> QSESYKDAYSRINAIVIEGEQEAFDNYNRLAEMLPDQRDELHKLAKMEQRHMKGFMACGKNLSVTPDMGFAQKFFERLHENFKAAAAEGKVVTCLLIQSLIIECFAIAAFNIYIPVADAFARKITEGVVRDEYLHRNFGEEWLKANFDASKAELEEANRQNLPLVWLMLNEVADDARELGMERESLVEDFMIAYGEALENIGFTTREIMRMSAYG;> SYKDAYSRINAIVIEGEQEAFDNYNRLAEMLPDQRDELHKLAKMEQRHMKGFMACGKNLSVTPDMGFAQKFFERLHENFKAAAAEGKVVTCLLIQSLIIECFAIAAFNIYIPVADAFARKITEGVVRDEYLHRNFGEEWLKANFDASKAELEEANRQNLPLVWLMLNEVADDARELGMERESLVEDFMIAYGEALENIGFTTREIMRMSAYG

Cyanobacterial aldehyde-deformylating oxygenase (cADO), which catalyzes the conversion of Cn fatty aldehyde to its corresponding Cn-1 alk(a/e)ne, is a key enzyme in that pathway. Cyanobacterial aldehyde-deformylating oxygenase (cADO) belongs to the superfamily of ferritin-like di-iron proteins and contains a di-iron center. To gain insights into the reaction catalyzed by cADO, we determined structures of wild type ADO from Synechococcus elongates PCC7942 (Se) with different treatment (WT0, no treatment; WT1, co-crystallized with iron; WT-HP, soaked in H2O2), and solved the structures of two SeADO mutants (Y122F and F86YF87Y). SeADO belongs to the di-iron protein family, with conserved sequence of two EX28-29EX2H motifs, in which six conservative amino acids from four helices (Glu32 from helix H1, Glu115 from helix H4, Glu60 & His63 from helix H2, and Glu144 & His147 from helix H5) act as metal ligands.

In the Y122F structure, very little electron density was observed in the substrate channel, which is in contrast to all other four structures. However, there is still a little electron density remaining in the vicinity of the di-iron site, which we assigned to a water molecule forming a hydrogen-bond interactions with the carboxylic oxygen atoms of Glu144 and Glu115. This water molecule is not coordinated to either iron ions, with a distance of 3.28 Å and 3.15 Å, respectively. Apart from harboring the vacant substrate channel, the Y122F mutant shows comparable enzymatic activity with wild type. This result is consistent with that of the equivalent Y135F mutant in PmADO. In the Y122F structure, the di-iron site is surrounded by the four-helix bundle, each iron ion is penta-coordinated by two bridging carboxylates ligands (Glu60 and Glu144), one bidentate carboxylates and one histidine ligand (Glu32 and His63 for Fe1, Glu115 and His147 for Fe2). The coordination geometry of the two iron atoms is similar to that of other di-iron proteins in their rest state of reduced forms which is consistent with the initial state of cADO in the reaction cycle.>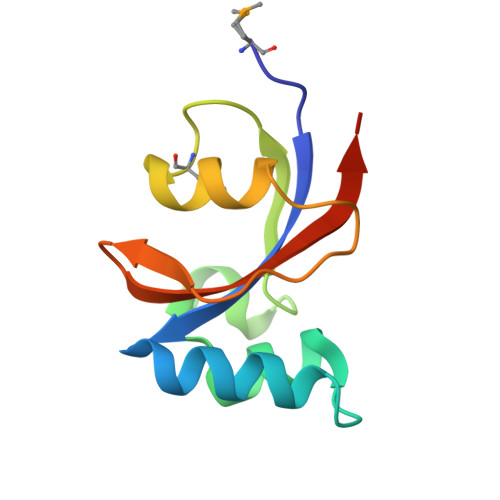[2x]MKPEIKASHILVKDEATAKKVKEELGQGKSFEELAKQYSEDTGSKEKGGDLGFFGAGKMVKEFEDAAYKLKKDEVSEPVKSQFGYHIIKVTDIENLYFQ> SNAMHNHNNRLVITPGEP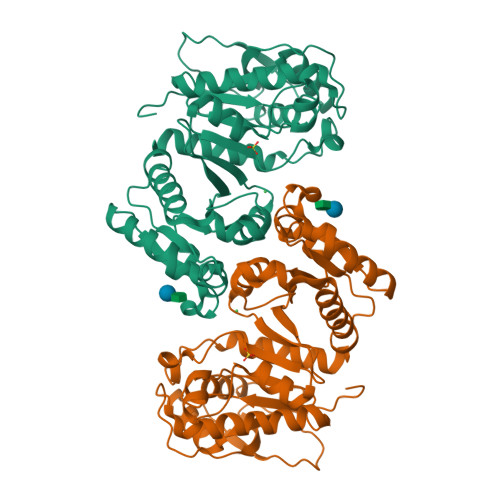AGVGPDLAITLAQQDWPVELVVCADPALLLARASQLNLPLQLREYQADQPAIAQQAGSLTILPVKTAVNVVPGKLDVGNSHYVVETLAKACDGAISGEFAALVTGPVQKSIINDAGIPFIGHTEFFADRSHCQRVVMMLATEELRVALATTHLPLLAVPGAITQASLHEVITILDNDLKTKFGITQPQIYVCGLNPHAGEGGHMGHEEIDTIIPALNTLRQQGINLIGPLPADTLFQPKYLQHADAVLAMYHDQGLPVLKYQGFGRAVNITLGLPFIRTSVDHGTALELAATGTADVGSFITALNLAIKMINNSNE>SLALSSPILKEILIEAPSYAPNSFTFDSTNKGFYTSVQDGRVMKYEGPNSGFV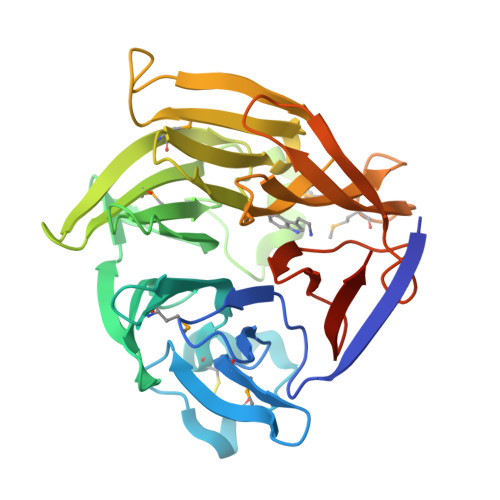DFAYASPYWNKAFCENSTDAEKRPLCGRTYDISYNLQNNQMYIVDCYYHLSVVGSEGGHATQLATSVDGVPFKWLYAVTVDQRTGIVYFTDVSTLYDDRGVQQIMDTSDKTGRLMKYDPSTKETTLLMKELHVPGGAEVSADSSFVLVAEFLSHQIVKYWLEGPKKGTAEVLVKIPNPGNIKRNADGHFWVSSSEELDGNMHGRVDPKGIKFDEFGNILEVIPLPPPFAGEHFEQIQEHDGLLYIGTLFHGSVGILVYDKKGNSFVSSH[2x]> IIGGTECKPHSRPYMAYLEIVTSNGPSKFCGGFLIRRNFVLTAAHCAGRSITVTLGAHNITEEEDTWQKLEVIKQFRHPKYNTSTLHHDIMLLKLKEKASLTLAVGTLPFPSQFNFVPPGRMCRVAGWGRTGVLKPGSDTLQEVKLRLMDPQACSHFRDFDHNLQLCVGNPRKTKSAFKGDSGGPLLCAGVAQGIVSYGRSDAKPPAVFTRISHYRPWINQILQAN

Chymase is a mast-cell-specific serine protease that is stored within secretory granules and released together with heparin and histamine in response to allergen challenge or other stimuli. Recent studies have shown that chymases possess processing activity for biological peptides and cytokines implicated in a variety of diseases. For example, the chymases of primates and dogs have highly specific angiotensin II (Ang II) generating activity, and the results of animal studies suggest that chymase contributes to the pathogenesis of cardiovascular diseases via Ang II generation. Based on the results of these studies, inhibition of chymase is expected to provide therapeutic means for the treatment of these diseases.

The crystal structure of human chymase with TJK002 was determined at 2.8 Å resolution. X-ray crystallographic study showed that TJK002 forms a non-covalent interaction with the catalytic domain of human chymase. The 4-methylbenzothiophen-3-yl fragment of TJK002 occupies the S1 pocket. The benzene ring of the benzimidazole scaffold shallowly occupies the S2 domain and could not form an effective hydrophobic interaction to the S2 site. The alkyl chain of S-butyric acid is bent and the carboxylic acid motif of TJK002 forms hydrogen bonds to the residues which are members of a catalytic triad (His57, Ser195). In our case the druglike carboxylic acid motif of TJK002 supplies two O atoms in the binding to the protein, which represent a new serine protease inhibitor motif. The carboxylic acid fragment of TJK002 forms hydrogen bonds with the imidazole N(∊) atom of His57 and/or the O(γ) atom of Ser195 which is a member of a catalytic triad. This imidazole ring of His57 forms π–π-stacking with the benzene ring of the benzimidazole scaffold as P2 moiety. Fragment molecular orbital (FMO) calculation of the atomic coordinates by X-ray crystallography showed that this imidazole ring of His57 could be protonated with the carboxyl group of Asp121 or the oxyanion group of Ser195 and the stacking interaction between the benzimidazole group and His57 is stabilized. So far the importance of the S2 site has not been noted, but this π–π interaction between the benzene ring of the benzimidazole scaffold inhibitor at the S2 site makes sense because the stacking interaction is also found in the complexes crystallized under different pH conditions.> CGACG;> CCCGC;> CG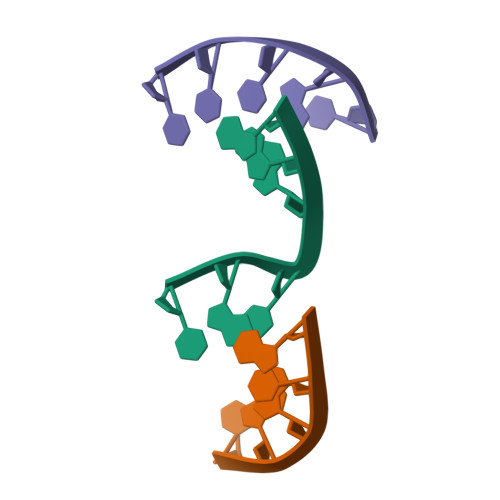TGGG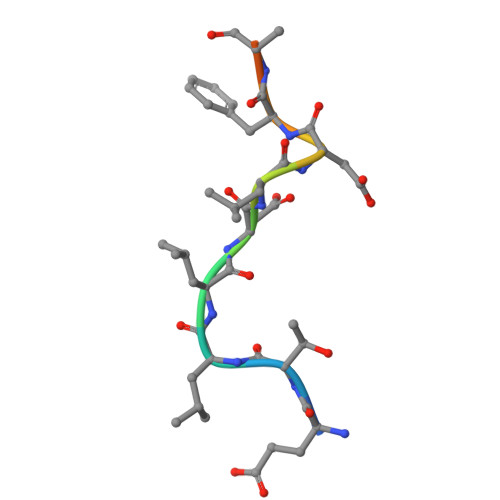> ETLLDLDFDPFK> MAEPVSPLKHFVLAKKAITAIFDQLLEFVTEGSHFVEATYKNPELDRIATEDDLVEMQGYKDKLSIIGEVLSRRHMKVAFFGRTSSGKSSVINAMLWDKVLPSGIGHITNCFLSVEGTDGDKAYLMTEGSDEKKSVKVNNQLAHALHMDKDLKAGCLVRVFWPKAKCALLRDDLVLVDSPGTDVTTELDSWIDKFCLDADVFVLVANSESTLMNTEKHFFHKVNERLSKPNIFILNNRWDASASEPEYME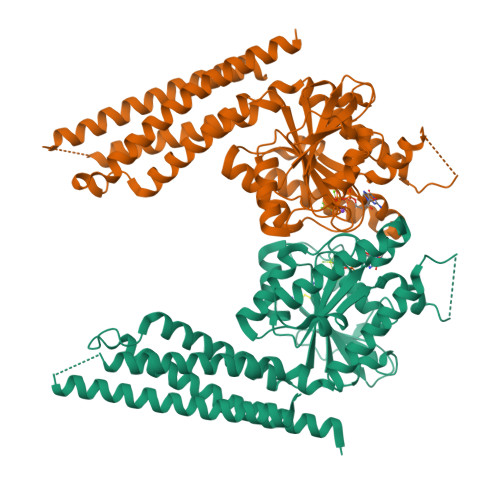DVRRQHMERCLHFLVEELKVVNALEAQNRIFFVSAKEVLSARKQKAQGMPESGVALAEGFHARLQEFQNFEQIFEECISQSAVKTKFEQHTIRAKQILATVKNIMDSVNLAAEDGSGSGSGGSEIARLPKEIDQLEKIQNNSKLLRNKAVQLENELENFTKQFLPSSNEES;>[2x]MAEPVSPLKHFVLAKKAITAIFDQLLEFVTEGSHFVEATYKNPELDRIATEDDLVEMQGYKDKLSIIGEVLSRRHMKVAFFGRTSSGKSSVINAMLWDKVLPSGIGHITNCFLSVEGTDGDKAYLMTEGSDEKKSVKTVNQLAHALHMDKDLKAGCLVRVFWPKAKCALLRDDLVLVDSPGTDVTTELDSWIDKFCLDADVFVLVANSESTLMNTEKHFFHKVNERLSKPNIFILNNRWDASASEPEYMEDVRRQHMERCLHFLVEELKVVNALEAQNRIFFVSAKEVLSARKQKAQGMPESGVALAEGFHARLQEFQNFEQIFEECISQSAVKTKFEQHTIRAKQILATVKNIMDSVNLAAEDGSGSGSGGSEIARLPKEIDQLEKIQNNSKLLRNKAVQLENELENFTKQFLPSSNEES> DNGGYVPAVVIGTGYGAAVSALRLGEAGVQTLMLEMGQLWNQPGPDGNIFCGMLNPDKRSSWFKNRTEAPLGSFLWLDVVNRNIDPYAGVLDRVNYDQMSVYVGRGVGGGSLVNGGMAVEPKRSYFEEILPRVDSSEMYDRYFPRANSMLRVNHIDTKWFEDTEWYKFARVSREQAGKAGLGTVFVPNVYDFGYMQREAAGEVPKSALATEVIYGNNHGKQSLDKTYLAAALGTGKVTIQTLHQVKTIRQTKDGGYALTVEQKDTDGKLLATKEISCRYLFLGAGSLGSTELLVRARDTGTLPNLNSEVGAGWGPNGNIMTARANHMWNPTGAHQSSIPALGIDAWDNSDSSVFAEIAPMPAGLETWVSLYLAITKNPQRGTF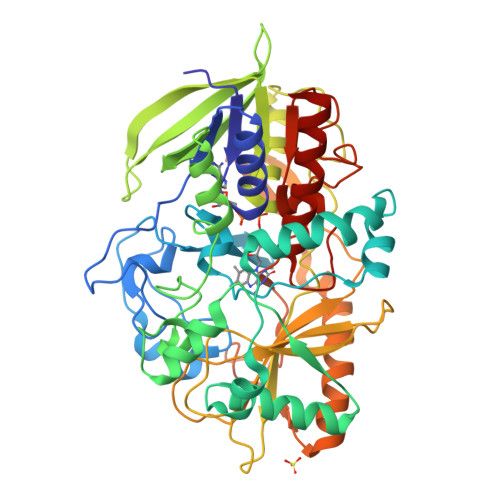VYDAATDRAKLNWTRDQNAPAVNAAKALFDRINKANGTIYRYDLFGTQLKAFADDFCYHPLGGCVLGKATDDYGRVAGYKNLYVTDGSLIPGSVGVDPFVTITALAERNVERIIKQDVTAS FKBP51 is the co-chaperone to Hsp90 and belongs to the immunophilin family initially recognized for its involvement in regulation of steroid hormone receptor activity. Going from the N-terminus to C-terminus, the overall FKBP51 structure contains two mixed beta sheet wrapped around a central helix for FK1 and FK2 domains followed by the TPR domain consisting of three TPR repeats and one additional long helix in the C-terminus. FK1 domain is active as PPIase and known to bind to the FK506 and rapamycin inhibitors or modulators. Inside the cell, the TPR domain of FKBP51 mediates interaction with EEVD C-terminal sequence of Hsp90/Hsp70 molecular chaperones.

We solved the crystal structure of both the native form of FKBP51 and in complexation with the C90 peptide. The elongated shape of FKBP51 leads to non-uniform crystal packing and therefore anisotropic order and diffraction from our crystals. During x-ray data collection we noticed that the diffraction pattern was quite anisotropic and therefore, decided to truncate the data in an ellipsoidal fashion using diffraction anisotropy server for the complex and the Staraniso software for the native structure. For the native, we used reflections up to 1.88 Å in elliptical shape with 93% completeness (52% completeness with spherical truncation) while standard spherical truncation would have resulted in a 2.45 Å resolution being 100% complete. The native structure has R and Rfree values of 0.198 and 0.247, respectively at the resolution of 1.88 Å (52% spherical completeness) while the complex structure has the R and Rfree values of 0.192 and 0.262, respectively at 2.49 Å (62% spherical completeness). Using secondary-structure matching (SSM) server, we compared the RMSD between our two structures and previously reported structure and found that the RMSD between native and the complex structure was 0.48 Å and the RMSD between native and previously reported structure was 0.49 Å while the RMSD between the complex and reported structure was found to be 0.61 Å for 349 aligned residues. The two native structures are more similar as compared to the complex structure. The structure of native FKBP51 is already reported at a resolution of 2.7 Å33.

> GPLGSMTTDEGAKNNEESPTATVAEQGEDITSKKDRGVLKIVKRVGNGEETPMIGDKVYVHYKGKLSNGKKFDSSHDRNEPFVFSLGKGQVIKAWDIGVATMKKGEICHLLCKPEYAYGSAGSLPKIPSNATLFFEIELLDFKGEDLFEDGGIIRRTKRKGEGYSNPNEGATVEIHLEGRCGGRMFDCRDVAFTVGEGEDHDIPIGIDKALEKMQREEQCILYLGPRYGFGEAGKPKFGIEPNAELIYEVTLKSFEKAKESWEMDTKEKLEQAAIVKEKGTVYFKGGKYMQAVIQYGKIVSWLEMEYGLSEKESKASESFLLAAFLNLAMCYLKLREYTKAVECCDKALGLDSANEKGLYRRGEAQLLMNEFESAKGDFEKVLEVNPQNKAARLQISMCQKKAKEHNERDRRIYANMFKKFAEQDAKEEANKAMGKKTSEGVTNEKGTDSQAMEEEKPEGHV> VAFGADAAKTTQEKFDALKEAGVFSGYPGTTDAKLGQDMTRAEFAKVLVKLFGLKEIHGQYSYKDKNYDAKNWAAPFIEAVTAEGLMQGKDLTKKIFDFNGKITVEEASKTLVTALKLEPVKDAQNKATDWAKGYFEAAVNAGLFSKDANPKAN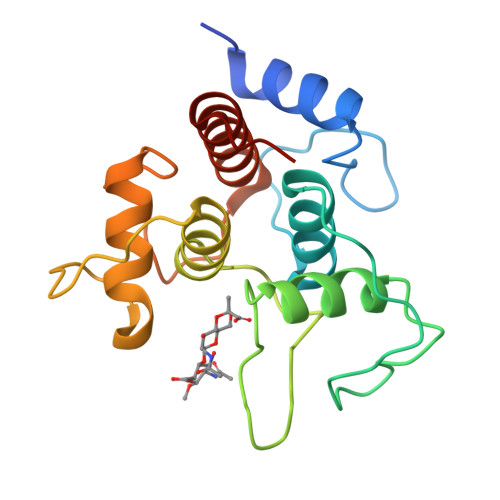ATRAQLVEAAFAADEMSKGSGSHHHHHH> DRASKIEQIQKLAKYAISALNYEDLPTAKDE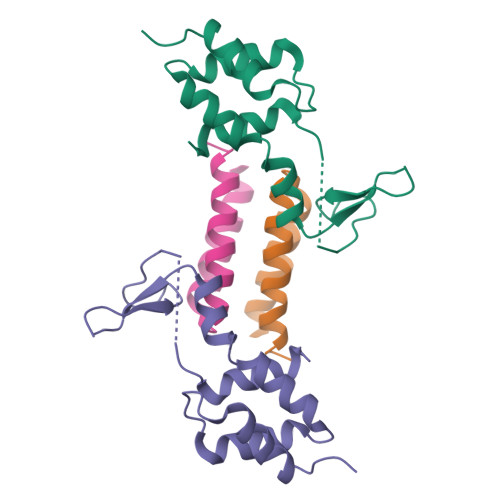LTKALDLLNSI;> GSPDLAARTTMFEINVGDTPCVLTKEDYRTLGAMTEGYSGSDIAVVVKDALMQPIRKIQSATHFKDVSTEDDETRKLTPCSPGDDGAIEMSWTDIEADELKEPDLTIKDFLKAIKST>GSAKDLMTLRSALLALLSSGPLTGYDASQRFGASVGFVWSGSDSQIYPELRKMEAEELLVGSDVPWGSKGATKTEYALSEKGWEALRKAWYEPVTYGPTRDPARLKAAYFEVGTNGDARRHLRAHIAHFEQQKIQSESMIDELKAKTHPTLARRLERSPKKEHERIVAFKVLAYEGQIARAQAEIEW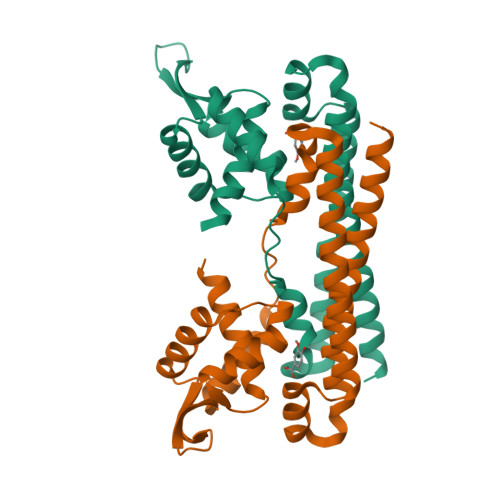AEKGLKLLDTL[2x]>[2x]MTMDEQQSQAVAPVYVGGFLARYDQSPDEAELLLPRDVVEHWLHAQGQGQPSLSVALPLNINHDDTAVVGHVAAMQSVRDGLFCLGCVTSPRFLEIVRRASEKSELVSRGPVSPLQPDKVVEFLSGSYAGLSLSSRRCDDVEQATSLSGSETTPFKAVALCSVGRRRGTLAVYGRDPEWVTQRFPDLTAADRDGLRAQWQRCGSTAVDASGDPFRSDSYGLLGNSVDALYIRERLPKLRYDKQLVGVTER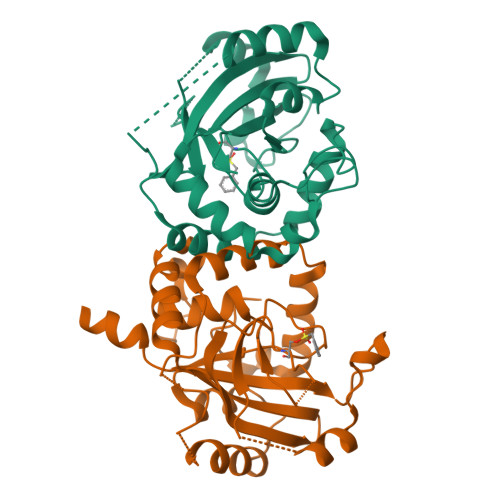ESYVKA> MEGLTIDLKNFRKPGEKTFTQRSRLFV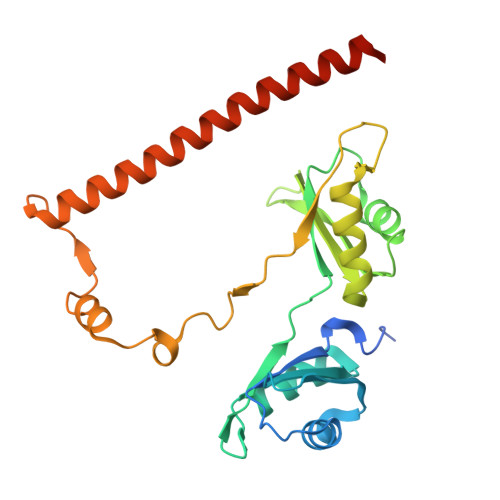GNLPPDITEEEMRKLFEKYGKAGEVFIHKDKGFGFIRLETRTLAEIAKVELDNMPLRGKQLRVRFACHSASLTVRNLPQYVSNELLEEAFSVFGQVERAVVIVDDRGRPSGKGIVEFSGKPAARKALDRCSEGSFLLTTFPRPVTVEPMDQLDDEEGLPEKLVIKNQQFHKEREQPPRFAQPGSFEYEYAMRWKALIEMEKQQQDQVDRNIKEAREKLEMEMEAARHEHQVMLM> MEAVLSRQAATAEAIGRFQDSSTSVGLVAGSPSTRIRRQADNVVLKSTSQAGDTLNDVIQDPTRRNKLINDNNLLKGIIMGRDGPVPSSRELIVRPDTLRAIINNRATIETTTMEAEFTETLMESNYNSASVKVSAPFITANSEYSESSSFKNTETEKSMYTSSRYLFPQGRIDFTTPDSGFDDVIKLSPQFTSGVQAALAKATGTEKREALQNLFQEYGHVFRTKVHIGGVLSAHTMETFSRSENETEVKQDVKAGLEGAVKGWGGGATAGHGNTQGTITTSQNRKLNVKYIVNGGDYTKIQNTEEWVASTNQSEHWRVIEVTEVTAVADLLPQPIRGQVKDLLKPLLGKWVDVEKVPGLESLPVSVYRPKGAIPAGWFWLGDTADASKALLVKPTLPARSGRNPALTSLHQGSGMTEQPFVDLPQYQYLSTYFGSFAHDTPPGSTLRGLRPDHVLPGRYEMHGDTISTAVYVTRPVDVPFPEDECFDLKSLV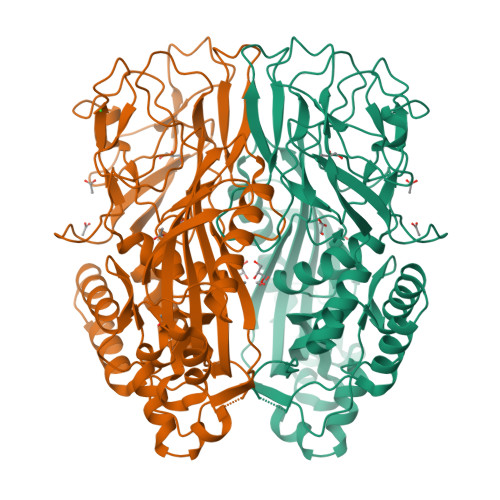RVKLPGSGNPPKPRSALKKSMVLFDSGEK>MSLQGIHLSDLSYKHAILKESQYTIKRDVGTTTAVTPSSLQQEITLLCGEILYAKHADYKYAAEIGIQYISTALGSERVQQILRNSGSEVQVVLTRTYSLGKIKNNKGEDLQMLDIHGVEKSWVEEIDKEARKTMATLLKESSGNIPQNQRPSAPDTPIILLCVGALIFTKLASTIEVGLETTVRRANRVLSDALKRYPRMDIPKIARSFYDLFEQKVYHRSLFIEYGKALGSSSTGSKAESLFVNIFMQAYGAGQTMLRWGVIARSSNNIMLGHVSVQAELKQVTEVYDLVREMGPESGLLHLRQSPKAGLLSLANCPNFASVVLGNASGLGIIGMYRGRVPNTELFSAAESYAKSLKESN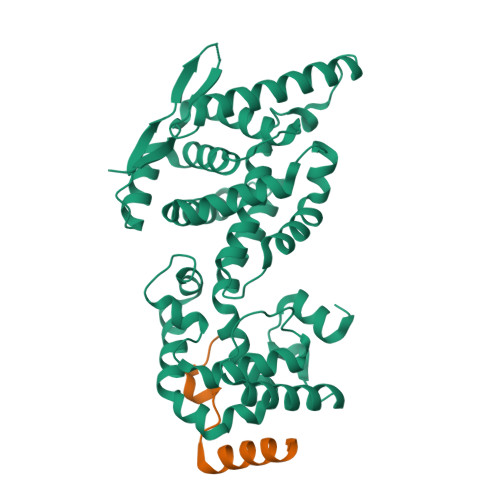KINFSSLGLTDEEKEAAEHFLNVSDDSQNDYE[2x];>[2x]MSFPEGKDILFMGNEAAKLAEAFQKSLRKPGHKRSQSIIGKHHHHHH Previous studies showed that proper introduction of disulfide bonds could stabilize the flexible region of target proteins and reduce the conformational entropy by locking the protein into single desired conformation. Here we developed a comprehensive disulfide bond prediction algorithm that not just increased the success rate of predictions but also improved the quality of crystallized target proteins. We applied our method on two proteins which were previously determined to high resolution and frequently used as fusion partners for GPCR crystallization, cytochrome b562 (BRIL) and Flavodoxin, and verified our prediction by solving the crystal structures of the wild type (WT) proteins and mutants. The theoretical and experimental results both indicated that with relatively lower values of conformational entropy, proteins would be more stable and readily crystallized to higher diffraction resolution.

The continued disulfide omitted electron densities of the side chains suggested that the disulfide bonds are successfully formed in all crystallized mutants, which are T9C-A36C, A20C-Q25C, V16C-A29C, and K27C-A79C in BRIL and N14C-C93, A43C-L74C, and C102-R125C in Flavodoxin, respectively. The WT and disulfide engineered Flavodoxin structures were determined to high-resolution of 1.20–1.55 Å with B-factors in the range of 16.15–19.24 Å2. A43 is located in a highly dynamic loop region and the disulfide bond A43C-L74C stabilized the loop region (the local B-factor decreased). For Flavodoxin, smaller fluctuations of the terminal distances suggest that A43C-74C is more stable among four proteins. On the other hand, the V16C-A29C and A20C-Q25C in BRIL, the N14C-C93 and A43C-L74C in Flavodoxin have higher entropy than that of WT counterparts, consistent with their relatively lower diffraction resolutions.

> SAKALIVYGSTTGNTEYTAETIARELADAGYEVDSRDAASVECGGLFEGFDLVLLGCSTWGDDSIELQDDFIPCFDSLEETGAQGRKVACFGCGDSSWEYFCGAVDAIEEKLKNLGAEIVQDGLRIDGDPRAARDDIVGWAHDVRGAI> MGLKLDLTWFDKSTEDFKGEEYSKDFGDDGSVMESLGVPF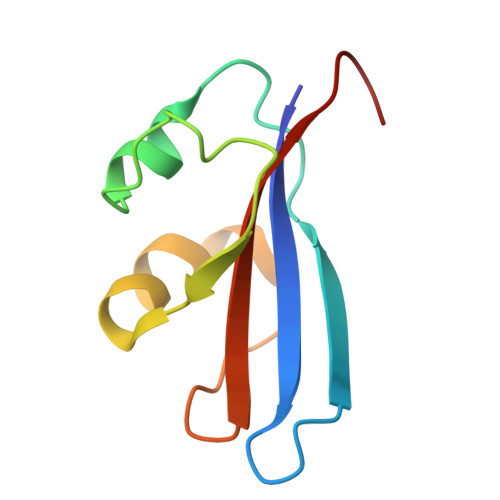KDNVNNGCFDVIAEWVPLLQPYFNHQIDISDNEYFVSFDYRDGDW>[2x]MGSSHHHHHHSSHMGEGQGPKKQTRLGLEAKKEENLADWYSQVITKSEMIEYHDISGCYILRPWAYAIWEAIKDFFDAEIKKLGVENCYFPMFVSQSALEKEKTHVADFAPEVAWVTRSGKTELAEPIAIRPTSETVMYPAYAKWVQSHRDLPIKLNQWCNVVRWEFKHPQPFLRTREFLWQEGHSAFATMEEAAEEVLQILDLYAQVYEELLAIPVVKGRKTEKEKFAGGDYTTTIEAFISASGRAIQGGTSHHLGQNFSKMFEIVFEDPKIPGEKQFAYQNSWGLTTRTIGVMTMVHGDNMGLVLPPRVACVQVVIIPCGITNALSEEDK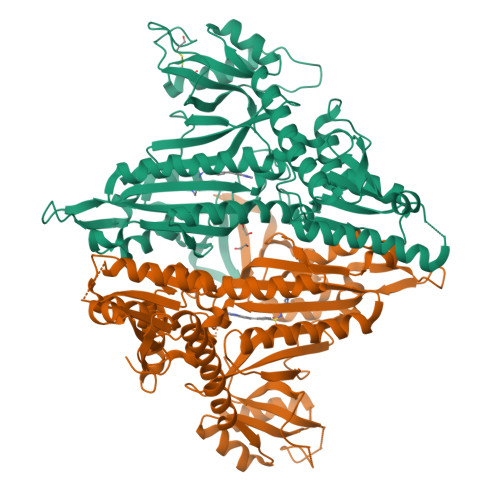EALIAKCNDYRRRLLSVNIRVRADLRDNYSPGWKFNHWELKGVPIRLEVGPRDMKSCQFVAVRRDTGEKLTVAENEAETKLQAILEDIQVTLFTRASEDLKTHMVVANTMEDFQKILDSGKIVQIPFCGEIDCEDWIKKTTARDQDLEPGAPSMGAKSLCIPFKPLCELQPGAKCVCGKNPAKYYTLFGRSY3-[2-[4-[[4-[2,2-bis(fluoranyl)-4,6,10,12-tetramethyl-1,3-diaza-2$l^{4}-boratricyclo[7.3.0.0^{3,7}]dodeca-4,6,9,11-tetraen-8-yl]phenoxy]methyl]-1,2,3-triazol-1-yl]ethyl]-1,5-dimethyl-6-[(1S)-2-oxidanyl-6-oxidanylidene-cyclohex-2-en-1-yl]carbonyl-quinazoline-2,4-dione 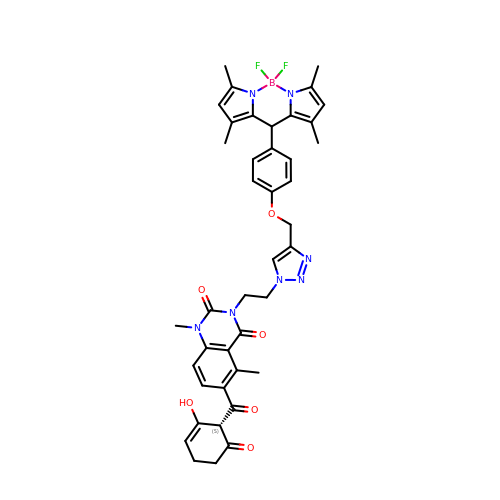| C41 H41 B F2 N7 O6 | DQUNZZSKKMECFQ-BHVANESWSA-N>ETGQVAASPSINVALKAAFPSPPYLVELLETAASDNTTIYYSLLDRIAKGHFAEATTDKALYEKFLEVLRDDGHMDPEALSAFKLALSLRTATPRVEAHYQYYTATVEPSLSGTQEGCDQWFLIDGEQYCSPTLDTSHGKVKGEDQLRTLPFDRKFGVGSRDVILYADITSKSFAPFHEVAMDLAKKGKASYRVRYRRSPSHSRESLSVNGYGVELVLKRTDYIVIDDRDTGAAAKPAEENDQKPLVGHETVLDDGEEIADIKPLEKSELAALGMKAASFVMQSEKPFEALLKLTQDFPKYSNSLGSQNVSAEFEAEHRGNREVFLPEGSNVLWLNGLHLIDRQIQPFGLVDLLTRERKLIKSVLDLGLTGQQAVDLLGHAEVAHAKSGDDEPRRFDWRDDIEEGQVIIWLNNLEKDKRYKSFSPSIWVLIHHFGHGLPQIRRDVFNLVVPVDLTKADDVKIVVEGLLSFVKRLIPVRFGFVPLTPTGQAIDQAKVVYYLLENYGLAAATAYLEKSYEEQSTGQPNERIFNEVIKDKSLRPDGVELSFKDIFISEKHEKQIHLSKHWVERLRAGGDVPTVFFDGFPIPREDNWLRVMNHRLMQDLQALQQAGYFGMLNESMWLPGFFLEKALSRRNTLIFPEDKNELTVLNVNKIYIENHDLMSKVPVIEASKESTRDDWAALTVVADLDDIEGQELVYYALRFRKSNDGVRLDIVHNPKDTSRSPSVLAQRLKSREDKLLDFTRFLDLETALETGEFEPDVAYDASLANFLASSNMKAGDNFVILNGRVLGPITSADDFKKEDFEVFLQAERRTRILPVYKALEDLGLDDKVSGPLSAAKLTSVTALSTISDLPQGIFDNAPTVRTTLFKQWNSTYTSFEVGDASTATIFFVAVINPASEIGQRWVAVLKVLSELEGVHLRV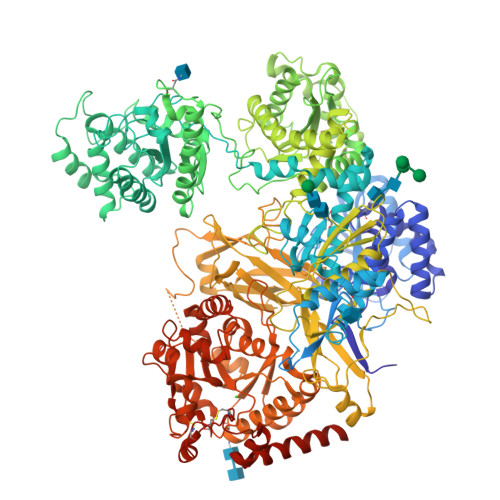FLNPTVMIEELPVKRFYRYVLSSSPSFDESGKVKALSARFTGVPRETLLVVGMDVPPAWLVTSKVAVDDLDNLRIKDIKAKRGTEHVEAIYELEHILIEGHSREIPGAHAPRGVQLVLETENNPHFADTIIMANLGYFQFKANPGVYNIRLKEGRSSEIFTLESVGAKGWGPIPGDDNTEVVLMDFQGTTLYPRLRRKPGMEEEDVLEPSTKSGEESGSGARNLVSRGIKFAEGLLGRGNKAAEATKSVSKTEHAEINIFSVASGHLYERMLNIMMASVMHHTNHTVKFWFIEQFLSPSFKDFIPHMAAEYGFKYEMVTYKWPHWLRQQKEKQREIWGYKILFLDVLFPLSLDKVIFVDADQIVRTDMYDLVEHPLDGAPYGFAPMCDSRVEMEGYRFWKTGYWANYLKGKPYHISALYVVDLQRFRELAAGDRLRQQYHALSADPNSLANLDQDLPNHMQFTIPIATLPQEWLWCETWCSDETLKDARTIDLCNNPMTKEPKLDRARRQVPEWTKYDEEIAELARRVREEKPKKKEEEKVQKNPKSRRLDGDEEEVKTVREGTKHHHHHH[2x]>KRKIIYLASPYGFSQQQKTLLLPPIVRALEALGIEVWEPFARNNQIDFSQADWAYRVAQADLQDVKNCDGIFAVVNGTPPDEGVMVELGMAIALNK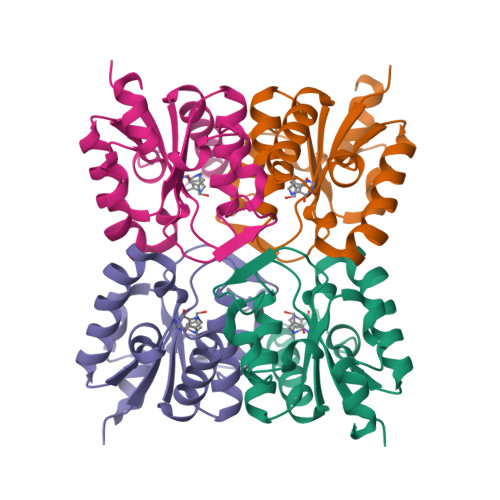AIFLFRDDFRRCSDNERYPLNLMLFAGLPEIGWENYYYTSVDEIQSHDKALYKWLTGM[4x]>MPNYKLTYFNMRGRAEIIRYIFAYLDIQYEDHRIEQADWPEIKSTLPFGKIPILEVDGLTLHQSLAIARYLTKNTDLAGNTEMEQCHVDAIVDTLDDFMSCFPWAEKKQDVKEQMFNELLTYNAPHLMQDLDTYLGGREWLIGNSVTWADF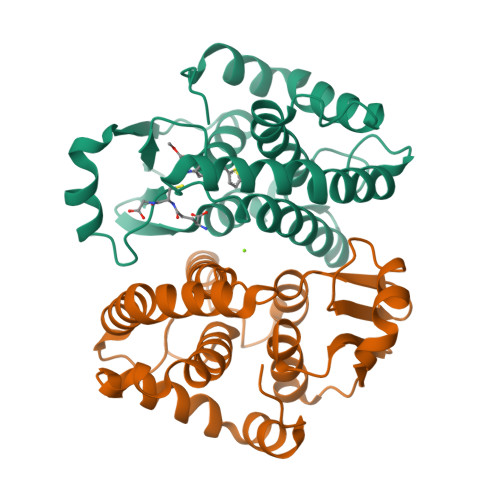YWEICSTTLLVFKPDLLDNHPRLVTLRKKVQAIPAIANWIKRRPQTKL[2x]> MKILVIEDDALLLQGLILAMQSEGYVCDGVSTAHEAALSLASNHYSLIVLDLGLPDEDGLHFLSRMRREKMTQPVLILTARDTLEDRISGLDTGADDYLVKPFALEELNARIRALLR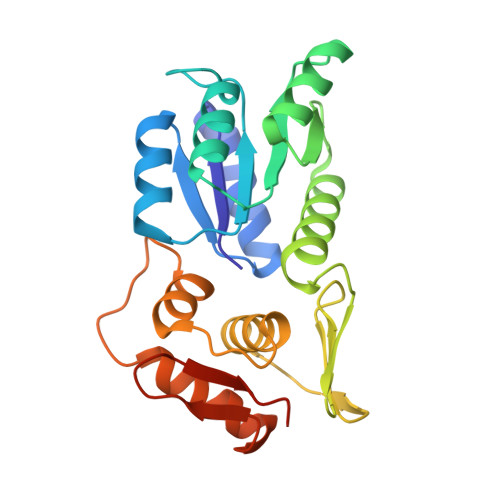RHNNQGDNEISVGNLRLNVTRRLVWLGETALDLTPKEYALLSRLMMKAGSPVHREILYNDIYSGDNEPATNTLEVHIHNLREKIGKSRIRTVRGFGYMLANNDDTEHLE>GL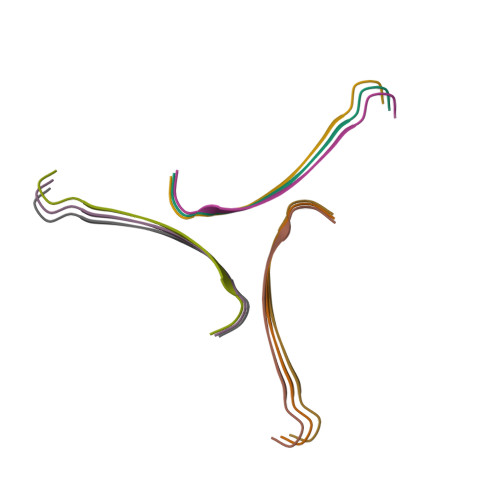FDIIKKVASVIGGL[9x]>PKLVLVRHGQSEWNEKNLFTGWVDVKLSAKGQQEAARAGELLKEKGVNVLVDYTSKLSRAIQTANIALEKADRLWIPVNRSWRLNERHYGDLQGKDKAQTLKKFGEEKFNTYRRSFDVPPPPIDASSPFSQKGDERYKYVDPNVLPETESLALVIDRLLPYWQDVIAKLVG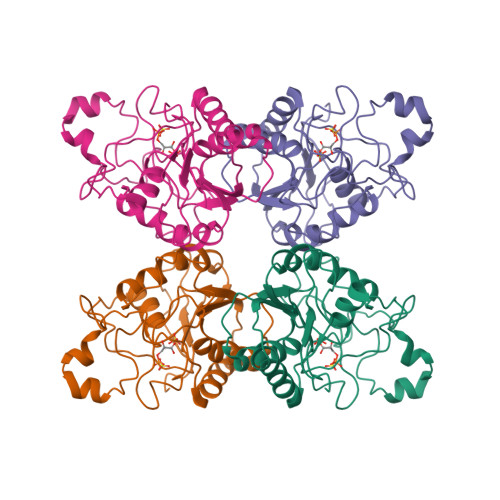KTSMIAAHGNSLRGLVKHLEGISDADIAKLNIPPGTILVFELDENLKPSKPSYYLDPEAAAAGAAAVANQGKK[2x]> MAIATYNSHVELAKYLVSKADSVYLTIGKSTPWSNETNPPQPDENATVLQEVIGYKKATKVTLVRPSKSPEDDNKNLI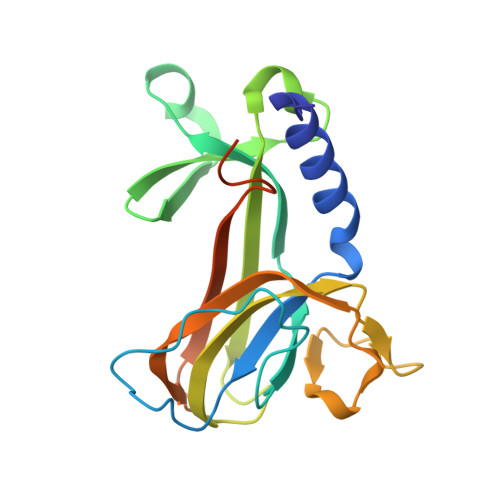SYGNKSWVEVTPENAKAEGAKWVYLESSIVGDELPLGTYRQVGFVMDLVAKSGISKFNLVPSEVESTGTLLFFDNKQFQNRSEQTTAKERFIVEVDPNSSSVDKLAAALEHHHHHH>QAQITGRPEWIWLALGTALMGLGTLYFLVKGMGVSDPDAKPFYAITTLVPAIAFTMYLSMLLGYGLTMVPFGGEQNPIYWARYADWLFTTPLLLLDLALLVDADQGTILALVGADGIMIGTGLVGALTKVYSYRFVWWAISTAAMLYILYVLFFGFTSKAESMRPEVASTFKVLRNVTVVLWSAYPVVWLIGSEGAGIVPLNIETLLFMVLDVSAKVGFGLILLRS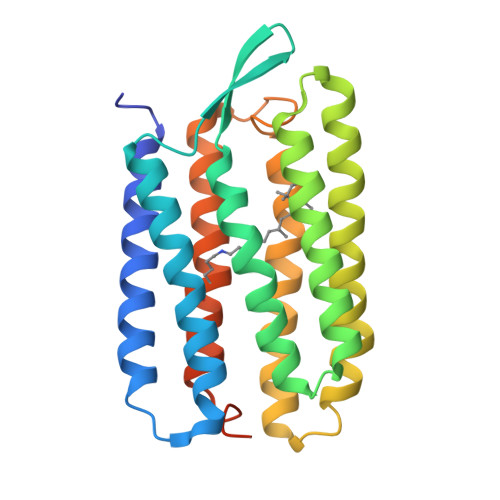RAIFGEAEAPEPSAGDGAAATSD[2x]> MTDKLIRELLIDVKQKGATRTAKSIENVSDALENAAAASELTNEQLGKMPKTLYSIERAADRAAKSLTKMQASRGMAGITKSIDSIGAKLDDLSIAMIEVADKLEAGFDGVSRSVKVMGNDVAAATEKVQDRLYDTNRVLGGTARGFNDTAGAAGRASRAIGNTSGSARGATRDFAAMAKVGGGLPLLYAAIASNIFVLQSAFEQLKLGDQLNRLEEFGVIVGTQTGTPVQSLARSLQEAAGYAISFEEAMRQASSASAYGFDAEQLNKFGLVARRAAAVLGVDMTDALNRVIKGVSKQEIELLDELGVTIRLNDAYADYVKQLNAANTGITYNINSLTTFQKQQAYANAVIAESTKRFGYLDEVLRATPWEQFAANADAALRTIQQAAAKYLGPVIDAINTVFYTSQA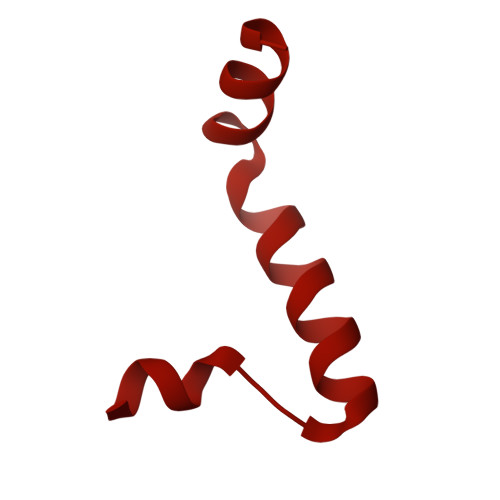SISAEAARAQEQTNKQIDPTNVGAVALSLSASEEGYNKALDMYKESLDKRNKLKSEFDKRMEQADFYTKLAIRQVGEGIPAGLATAGASEANKKFVEETAAMGLQVARLDKEVTDSTENLNAWKSAYQAAGAAAAKANPEFQKQINLQRDTTDPGAVYDFNSTVLKGLTEQQKAYNQTKKTASDLANDIQNVAQNTDTAAKTSATLADAIKNIESLSLGTGKSADEYVKNLNLGYNTLSEMKTASQALSEYVKLTGNETKNQLAVQQKIADVYNQTKDKEKAQEAGRRLELQQLEEQEAALRRVLQTNQGNKAVEREIEKIQLEKIKLTNQGMEAQKKVKDYTDKILGVDREIALLNNRTMTDTQYRLAQLNLELTIEKEKYEWYTKQADKQKEAEQSRRAQAQIEREIWKFHQDQQAEMTSKRQEAFENTLTSMFPLAGEMQKMEMQLDFYTQMKELTKDNANEQMRWNAEIAKTRAQMSALTAQRNAQMQSSVGSSLGAVYTPTTGLSGEDKKFADMGNQLASYDQAISKLSELNSEATAVAQSMGNLANAMIQFSQGSLDTTSTIAVGMQTVASMIQYSTSQQVSAIDQAIAAEQKRDGKSEASKAKLKKLEAEKLKIQQDAAKKQIIIQTAVAVMQAATAVPYPFSIPLMIAAGLAGALALAQASSASGMSSIGDSGADTASYLTLGERQKNIDVSMSANAGELSYVRGDKGIGNANSFVPRAEGGNMYPGVSYQMGEHGTEVVTPMVPMKATPNDELKNSSNSTAGRPIILNISAMDAASFREFASSNSGALRDAVELALNENGASLKTLGNS> SDHVE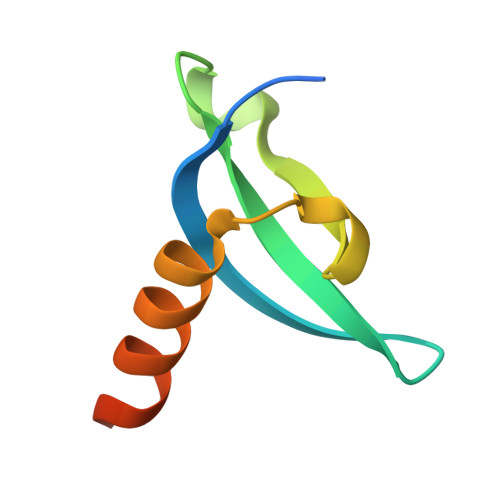EYVVEKILGKRFVNGRPQVLVKWSGFPNENNTWEPLENVGNCMKLVSDFESEVFRLHRKAAAK> MS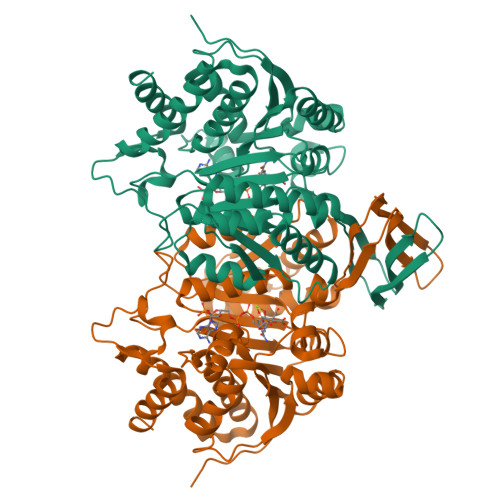KIKMKVPLVEMDGDEMTRIIWRLIKENLLEPYIELNTEYYDLGLENRDKTEDQVTIDAARAIQKYGVGVKCATITPNAQRVEEYNLKKMWKSPNGTIRAILDGTVFRAPIVVNSIKPFVKGWKKPISIARHAYGDVYKNVEYYVPSAGKAELVFTSENGEVSRQTIHEFDGPGVIMGMHNTDKSIRSFARACFNYALDMNQDLWFSTKDTISKTYDHRFKDIFQEIYENEYKEKFEAKNLQYFYTLIDDAVARIIRSEGGMVWACKNYDGDVMSDMVASAFGSLAMMTSVLVSPDGKYEFEAAHGTVTRHYYKHLKGEETSTNSMATIFAWTGALKKRGELDGIKELVDFATKLEQASVQTIENGVMTKDLASLSEVPEKKIVNTEDFLKEIRKTFEGMA>[2x]MERVLIVNADDFGLSKGQNYGIIEACRNGVVTSTTALVNGAAIDHAAQLGRSTP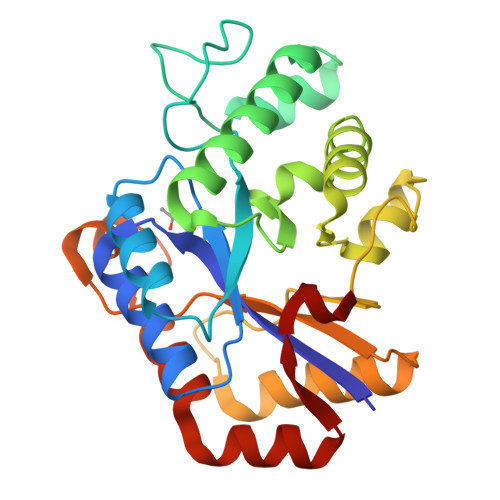ELAVGMHFVLTLGEPLSAMPGLTRDGRLGKWIWQQAEEDSLPLEEIAHELACQYHRFVELFGHEPTHIDSHHHVHMFAQIYPIVAAFAREKGIALRIDRQVAAQSGLDQQAARSSAGFSSEFYGEAVSEELFLQTLDASIARGERSLEVMCHPAYVDRIIMGSAYCYPRLDELDVLTAASLKAAVADRGYRLGTYRDVLE~{N}4-[3-(aminomethyl)phenyl]-1~{H}-indole-2,4-dicarboxamide 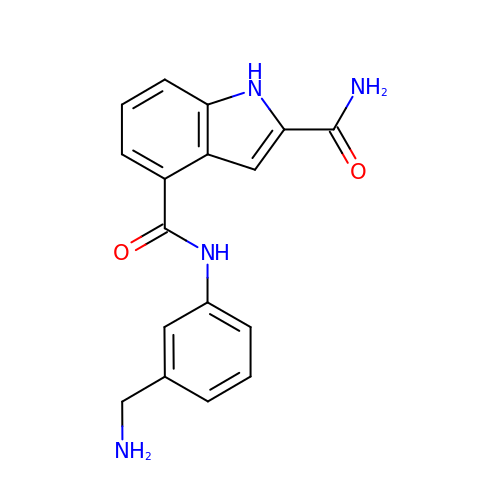| C17 H16 N4 O2 | BDFMFQJHWMAJCS-UHFFFAOYSA-N>GQGKLISVKTDVLDLTINTRGGDVEQALLPAYPKELNSTQPFQLLETSPQFIYQAQSGLTGRDGPDNPANGPRPLYNVEKDAYVLAEGQNELQVPMTYTDAAGNTFTKTFVLKRGDYAVNVNYNVQNAGEKPLEISSFGQLKQSITLPPHLDTGSSNFALHTFRGAAYSTPDEKYEKYKFDTIADNENLNISSKGGWVAMLQQYFATAWIPHNDGTNNFYTANLGNGIAAIGYKSQPVLVQPGQTGAMNSTLWVGPEI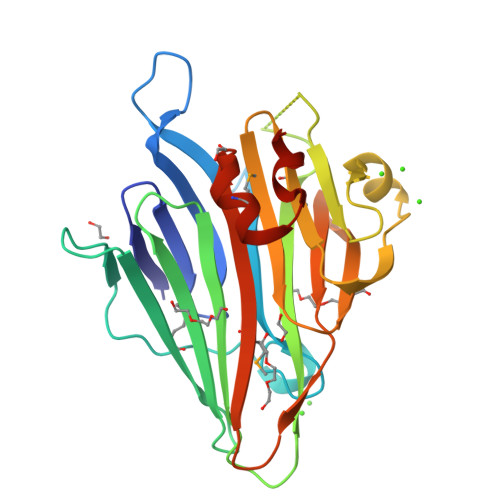QDKMAAVAPHLDLTVDHHHHHH[2x]> LPTSNPAQELEARQLERTTRDDLINGNSASCADVIFIYARGSTETGNLGTLGPSIASNLESAFGKDGVWIQGVGGAYRATLGDNALPRGTSCAAI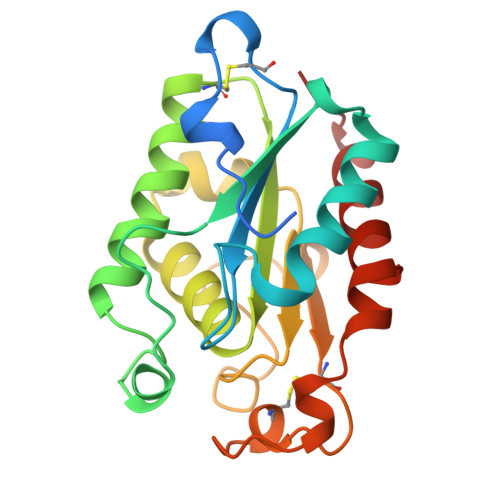REMLGLFQQANTKCPDATLIAGGYSQGAALAAASIEDLDSAIRDKIAGTVLFGYTKNLQNRGRIPNYPADRTKVFCNTGDLVCTGSLIVAAPHLAYGPDARGPAPEFLIEKVRAVRGSA>[2x]SAEIQPRSDEKRILSNVAVLEGAPPLSEHWQLFNNNEVLFNEARTAQAATVVFSLQQNAQIEPLARSIHTLRRQRGSAMKILVRENTASLRATDERLLLACGANMVIPWNAPLSRCLTMIESVQGQKFSRYVPEDITTLLSMTQPLKLRGFQKWDVFCNAVNNMMNNPLLPAH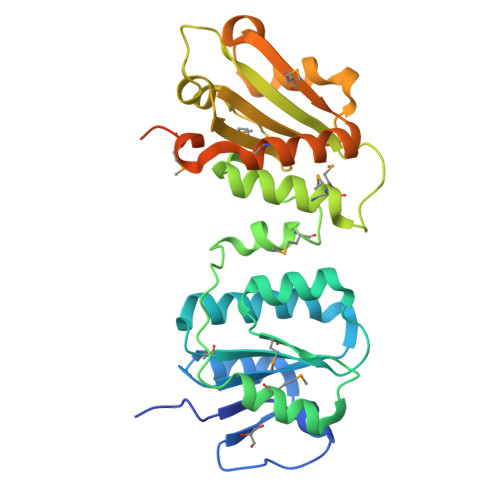GKGVLVALRPVPGIRVEQALTLCRPNRTGDIMTIGGNRLVLFLSFCRINDLDTALNHIFPLPTGDIFSNRMVWFEDDQISAELVQMRLLAPEQWGMPLPLTQSSKPVINAEHDGRHWRRIPEPMRLLDDAVERSS In this study, we used alkaline D-peptidase from Bacillus cereus DF4-B (ADP), an AmpH-type class C PBP141516, as a model for determining the peptide ligand recognition mechanism of PBPs. ADP acts as a D-stereospecific endopeptidase14 and degrades D-phenylalanine tetrapeptide [(D-Phe)] into dipeptides [(D-Phe)]14. ADP also catalyzes synthesis of peptides: for example, it can synthesize D-Phe oligopeptides from D-phenylalanine methyl ester. Residues from these motifs form a Ser/Tyr/His/Lys catalytic tetrad that dominates the catalysis of AmpH-type class C PBPs. This tetrad is also present in ADP (Ser74/Tyr171/His312/Lys77).

The crystal structure of the ADP (apo) form was determined at 2.1 Å resolution. The space group is P3221, and one ADP molecule is present in each asymmetric unit. The crystal structure of ADP consists of two subdomains: a five-stranded β-sheet flanked by three α-helices, and a cluster of mixed 310-helices and α-helices. A cavity for binding substrate peptides is also present near the active-site residues. Two regions, the Ω loop and the 283–293 loop (red circle), had higher B-factor values than the average value for the structure overall (32.2 Å2): the values for Ω loop and 283–293 loop are 73.9 and 56.7 Å2, respectively. Therefore, in this study, the ADP structure was compared with DD-peptidase. Three regions, the 132–144 loop, Ω loop, and 283–293 loop, have different conformations in the two proteins. In particular, the structure of the 132–144 loop of ADP is clearly different from that of DD-peptidase: in ADP, this region consists of 13 amino acids and has a loop structure (green), whereas in DD-peptidase it consists of 18 amino acids and contains a helix-turn-helix motif (orange). The catalytic tetrad of ADP is conserved in AmpH-type class C PBPs such as DD-peptidase7 and DAA9, and an oxyanion hole formed by the backbone amide N atoms of Ser74 and Ser315 is also present. Trp233 of DD-peptidase, which creates a small hydrophobic space required for accommodating a part of the side chain of D-Ala (P1) of the substrate (glycyl-L-α-amino-ε-pimelyl-D-Ala-D-Ala [REX]), is replaced by Met245 in ADP; this replacement creates the hydrophobic space required to accommodate a part of the D-Phe (P1) side chain of the ADP substrate. Initially, ADP forms a closed state in which the 132–144 and Ω loops interact.

> MKTRSQITCASLALLIAGSSLLYTTQTLIVKAEPTQSVSSSVQTSTQRDRNSVKQAVRDTLQLGFPGILAKTSEGGKTWSYAAGVANLSSKKPMKTDFRFRIGSVTKTFTATVVLQLAEENRLNLDDSIEKWLPGVIQGNGYDDKQITIRQLLNHTSGIAEYTRSKSFDLMDTKKSYRAEELVKMGISMPPDFAPGKSWSYSNTGYVLLGILIETVTGNSYAEEIENRIIEPLELSNTFLPGNSSVIPGTKHARGYIQLDGASEPKDVTYYNPSMGSSAGDMISTADDLNKFFSYLLGGKLLKEQQLKQMLTTVPTGEAALGRYGLGIYETKLPNGVSIWGHGGSIPGFVTFAGGTLGGKHTLAVNLNSLNAESPDPFKNILLAEFSK> MMHLKNIKSENPKTKEQYQLTKNFDVIWLWSEDGKNWYEEVNNFQDDTIKIVYDENNIIVAITKDASTLNPEGFSVVEIPDITANRRADDSGKWMFKDGAVVKRIYTADEQQQQAESQKAALLSEAESVIQ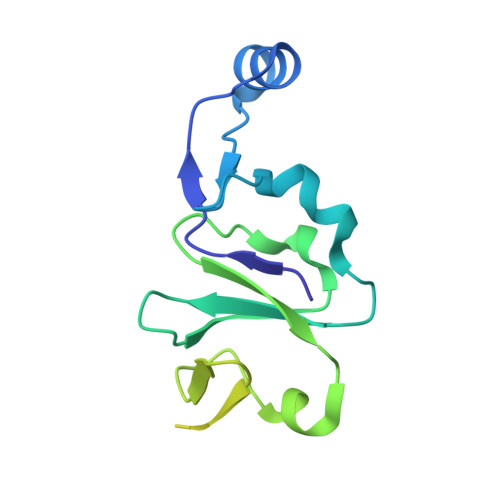PLERAVRLNMATDEERARLESWERYSVLVSRVDTANPEWPQKPE>[2x]MLRLDTRFLPGFPEALSRHGPLLEEARRRLLAKRGEPGSMLGWMDLPEDTETLREVRRYREANPWVEDFVLIGIGGSALGPKALEAAFNESGVRFHYLDHVEPEPILRLLRTLDP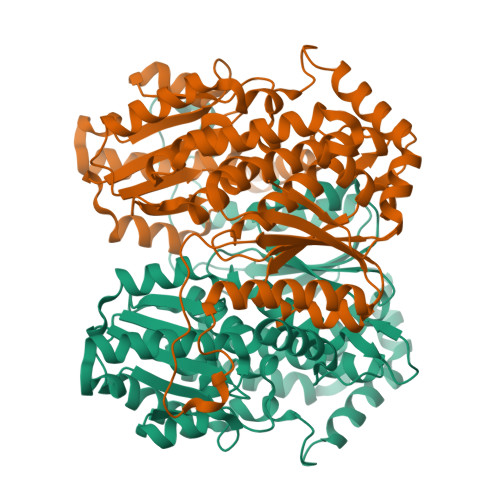RKTLVNAVSKSGSTAETLAGLAVFLKWLKAHLGEDWRRHLVVTTDPKEGPLRAFAEREGLKAFAIPKEVGGRFSALSPVGLLPLAFAGADLDALLMGARKANETALAPLEESLPLKTALLLHLHRHLPVHVFMVYSERLSHLPSWFVQLHDESLGKVDRQGQRVGTTAVPALGPKDQHAQVQLFREGPLDKLLALVIPEAPLEDVEIPEVEGLEAASYLFGKTLFQLLKAEAEATYEALAEAGQRVYALFLPEVSPYAVGWLMQHLMWQTAFLGELWEVNAFDQPGVELGKVLTRKRLAG4-[(6-CHLORO-2-NAPHTHALENYL)SULFONYL]-1-[[4-HYDROXYMETHYL-1-(4-PYRIDINYL)-4-PIPERIDINYL]METHYL]PIPERAZINONE 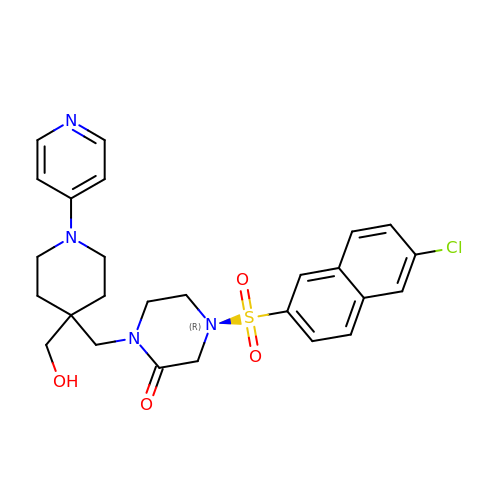| C26 H29 Cl N4 O4 S | ZRGAURKJCJQBQS-UHFFFAOYSA-N> GSKKLINDVQDVLDEQLAGLAKAHPSLTLHQDPVYVTRADAPVAGKVALLSGGGSGHEPMHCGYIGQGMLSGACPGEIFTSPTPDKIFECAMQVDGGEGVLLIIKNYTGDILNFETATELLHDSGVKVTTVVIDDDVAVKDSLYTAGRRGVANTVLIEKLVGAAAERGDSLDACAELGRKLNNQGHSIGIALGACTVPAAGKPSFTLADNEMEFGVGIHGEPGIDRRPFSSLDQTVDEMFDTLLVNGSYHRTLRFWDYQQGSWQEEQQTKQPLQSGDRVIALV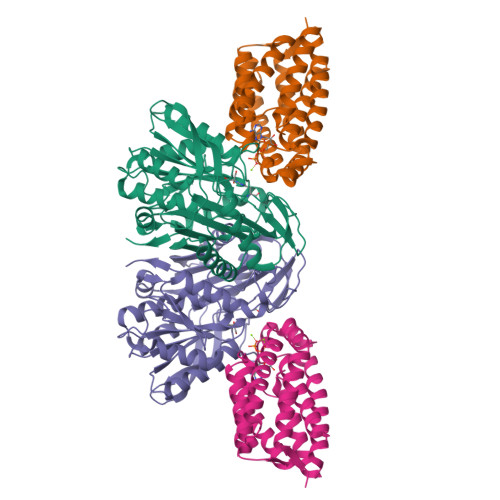NNLGATPLSELYGVYNRLTTRCQQAGLTIERNLIGAYCTSLDMTGFSITLLKVDDETLALWDAPVHTPALNWGK;> GSSLSRTQIVNWLTRCGDIFSTESEYLTGLDREIGDADHGLNMNRGFSKVVEKLPAIADKDIGFILKNTGMTLLSSVGGASGPLFGTFFIRAAQATQARQSLTLEELYQMFRDGADGVISRGKAEPGDKTMCDVWVPVVESLRQSSEQNLSVPVALEAASSIAESAAQSTITMQARKGRASYLGERSIGHQDPGATSVMFMMQMLALAAKE5,6-bis(fluoranyl)-3-(4-piperazin-1-yl-2-propan-2-yloxy-phenyl)-1~{H}-indole-2-carboxamide | C22 H24 F2 N4 O2 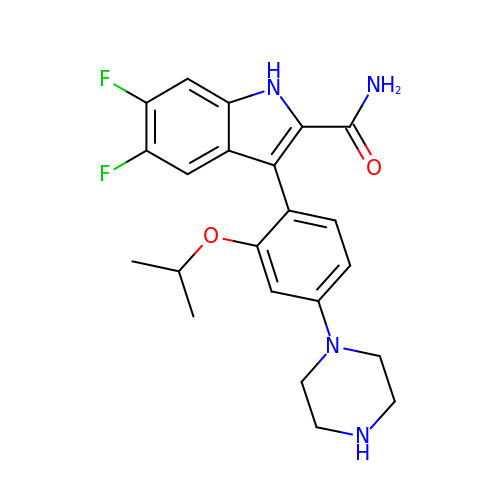| VLTSNEYKDGRFDU-UHFFFAOYSA-N>[3x]MKALEFQGPPMLPRPSGTYAGLPIADYGDAPPLSTKTMFWRTSPEKLPPGAWEPAYLGSKDERVDGPSLQQVMRDQLKPYSEPRGLLPPQEILDAVCDAIENRLENTLEPQKPWTFKKACESLDKNTSSGYPYHKQKSKDWTGSAFIGDLGDQATHANNMYEMGKSMR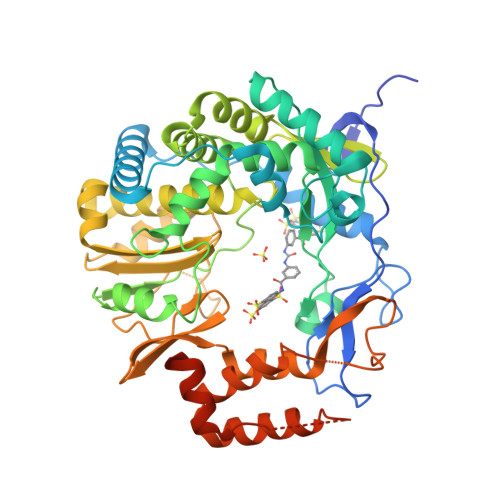PIYTAALKDELVKPDKIYGKIKKRLLWGSDLGTMIRAARAFGPFCDALKETCIFNPIRVGMSMNEDGPFIFARHANFRYHMDADYTRWDSTQQRAILKRAGDIMVRLSPEPDLARVVMDDLLAPSLLDVGDYKIVVEEGLPSGCPCTTQLNSLAHWILTLCAMVEVTRVDPDIVMQESEFSFYGDDEVVSTNLELDMVKYTMALRRYGLLPTRADKEEGPLERRQTLQGISFLRRAIVGDQFGWYGRLDRASIDRQLLWTKGPNHQNPFETLPGHAQRPSQLMALLGEAAMHGEKYYRTVASRVSKEAAQSGIEMVVPRHRSVLRWVRFGTMDAETPQERSAVFVNEDELEHHHHHH> MGHHHHHHHHHHSSGHIEGRHMLRERTVRLQYGSRVEAVYVLGTYLWTDVYSAAPAGAQTFSLKHSEHVWVEVVRDGEAEEVATNGKQRWLLSPSTTLRVTMSQASTEASSDKVTVNYYDEEGSIPIDQAGLFLTAIEISLDVDADRDGVVEKNNPKKASWTWGPEGQGAILLVNCDRETPWLPKEDCRDEKVYSKEDLKDMSQMILRTKGPDRLPAGYEIVLYISMSDSDKVGVFYVENPFFGQRYIHILGRRKLYHVVKYTGGSAELLFFVEGLCFPDEGFSGLVSIHVSLLEYMAQDIPLTPIFTD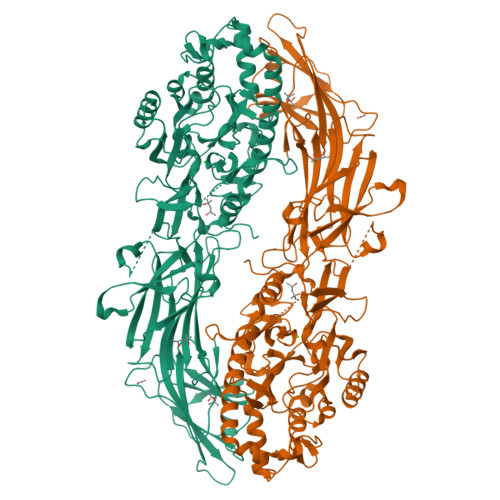TVIFRIAPWIMTPNILPPVSVFVCCMKDNYLFLKEVKNLVEKTNCELKVCFQYLNRGDRWIQDEIEFGYIEAPHKGFPVVLDSPRDGNLKDFPVKELLGPDFGYVTREPLFESVTSLDSFGNLEVSPPVTVNGKTYPLGRILIGSSFPLSGGRRMTKVVRDFLKAQQVQAPVELYSDWLTVGHVDEFMSFVPIPGTKKFLLLMASTSACYKLFREKQKDGHGEAIMFKGLGGMSSKRITINKILSNESLVQENLYFQRCLDWNRDILKKELGLTEQDIIDLPALFKMDEDHRARAFFPNMVNMIVLDKDLGIPKPFGPQVEEECCLEMHVRGLLEPLGLECTFIDDISAYHKFLGEVHCGTNVRRKPFTFKWWHMVPSRRS> MKDDLDNNLLYRYCGATSPFWRLPLDSNALQLAASEEAVTSHVVPLTPEQAAQIRTMSVITSSVTLSLSLFGELVPVHLVGRKVSRKEWAGTASA

DSFs are a family of fatty acid AIs produced and detected by a wide range of gram-negative bacteria, including important pathogens. The DSF receptor RpfR is conserved in numerous gram-negative bacteria, including, among others, Escherichia coli, B. cenocepacia, Cronobacter turicensis, Serratia marcescens, Yersinia enterocolitica, and Enterobacter cloacae. RpfR was predicted to contain three domains, namely Per-Arnt-Sim (PAS), diguanylate cyclase (DGC), and phosphodiesterase (PDE) domains. BDSF binding to RpfR was previously shown to trigger its PDE activity, decreasing the intracellular concentration of c-di-GMP and favoring biofilm dispersal.

We observed that the undescribed region of RpfR (residues 1–117) was highly conserved among all RpfR homologues. Indeed, we found that a construct containing the first 95 residues of RpfRCt (RpfRCt) was soluble and well folded, as determined by size exclusion chromatography. We determined the X-ray crystal structure of the RpfRCt(1–95) to a resolution of 1.2 Å using the single-wavelength anomalous dispersion (SAD) method. RpfRCt(1–95) adopts a Profilin-like fold consisting of an N-terminal α-helix and a central six-stranded antiparallel β-sheet with a single α-helix connecting β3 to β4. Distance-matrix alignment (DALI) and PDBeFold searches of the Protein Data Bank (PDB) show the closest RpfRCt(1–95) structural homologues to be PAS, Ca2+channels-chemotaxis receptors (Cache), and cyclic GMP-specific phosphodiesterase-adenylyl cyclase-FhlA (GAF) domains; however, canonical PAS domains contain five-stranded β-sheets, and Cache domains are periplasmic domain proteins that contain an additional N-terminal α-helix that extends through the membrane. Like RpfRCt(1–95), GAF domains contain six-stranded antiparallel β-sheets; however, unlike GAF domain proteins, RpfRCt(1–95) does not possess a pair of interacting α-helices below its β-sheet. Consistent with the fact that RpfRCt(1–95) is neither a PAS, Cache, or GAF domain, protein BLAST (BLASTP) searches using the RpfRCt(1–95) and RpfRBc(1–94) amino acid sequences return neither PAS, Cache, nor GAF domain proteins. Based on the above structural and sequence analysis, we conclude that while the RpfR N-terminal domain is structurally similar to PAS, Cache, and GAF domains, it is a new domain with a Profilin-like fold. As detailed below, this RpfR domain binds to and negatively regulates RpfF; thus, we refer to it as the RpfF interaction (FI) domain. Finally, superposing the structures of RpfRCt(FI) alone with the structure of RpfRCt(FI) in complex with RpfFBc reveals that RpfRCt(FI) undergoes minor conformational changes primarily at the RpfFBc binding surface.>[2x]MSEFNITETYLRFLEEDTEMTMPIAAIEALVTLLRIKTPETAAEMINTIKSSTEELIKSIPNSVSLRAGCDIFMRFVLRNLHLYGDWENCKQHLIENGQLFVSRAKKSRNKIAEIGVDFIADDDIILVHGYSRAVFSLLNHAANKFIRFRCVVTESRPSKQGNQLYTLLEQKGIPVTLIVDSAVGAVIDKVDKVFVGAEGVAESGGIINLVGTYSVGVLAHNARKPFYVVTESHKFVRMFPLSSDDLPMAGPPLDFTRRTDDLEDALRGPTIDYTAQEYITALITDLGVLTPSAVSEELIKMWYD;>[2x]MSSQAFTSVHPNAATSDVNVTIDTFVAKLKRRQVQGSYAIALETLQLLMRFISAARWNHVNDLIEQIRDLGNSLEKAHPTAFSCGNVIRRILAVLRDEVEEDTMSTTVTSTSVAEPLISSMFNLLQKPEQPHQNRKNSSGSSSMKTKTDYRQVAIQGIKDLIDEIKNIDEGIQQIAIDLIHDHEILLTPTPDSKTVLKFLITARERSNRTFTVLVTEGFPNNTKNAHEFAKKLAQHNIETLVVPDSAVFALMSRVGKVIIGTKAVFVNGGTISSNSGVSSVCECAREFRTPVFAVAGLYKLSPLYPFDVEKFVEFGGSQRILPRMDPRKRLDTVNQITDYVPPENIDIYITNVGGFNPSFIYRIAWDNYKQIDVHLDKNKA;>[2x]MSIQAFVFCGKGSNLAPFTQPDFPFQTQNKDSTAATSGDKLNELVNSALDSTVINEFMQHSTRLPKALLPIGNRPMIEYVLDWCDQADFKEISVVAPVDEIELIESGLTSFLSLRKQQFELIYKALSNSNHSHHLQDPKKINFIPSKANSTGESLQKELLPRINGDFVILPCDFVTDIPPQVLVDQFRNRDDNNLAMTIYYKNSLDSSIDKKQQQKQKQQQFFTVYSENEDSERQPILLDVYSQRDVTKTKYLQIRSHLLWNYPNLTVSTKLLNSFIYFCSFELCQLLKLGPQSMSRQASFKDPFTGNQQQQNPPTTDDDEDRNHDDDDDYKPSATSIQPTYFKKKNDLILDPINCNKSLSKVFRDLSRRSWQHSKPREPIGIFILPNETLFIRANNLNAYMDANRFVLKIKSQTMFTKNIQIQSAAIGADAIVDPKCQISAHSNVKMSVLGTQANIGSRCRVAGSLLFPGVHLGDEVILENCIIGPMAKIGSKCKLSNCYIEGHYVVEPKNNFKGETLANVYLDEDEEDELIYDDSVIAGESEIAEETDSDDRSDEDSDDSEYTDEYEYEDDGLFER;>MSESEAKSRSATPPSKAKQATPTTTAAANGEKKLTNKELKELKKQEKAAKRAAMKQANGISIEQQQQQAQMKKEKKQLQREQQQKREQKQKNANKKKQNERNVKKSTLFGHLETTEERRATILALTSAVSSPKTSRITAAGLMVPVVASALSGSNVLTASSLMPVGPNASSTVSASAPASTTTTLPASSAALSAGTSSASTNTPTAIQQEIASSNASDVAKTLASISLEAGEFNVIPGISSVIPTVLEQSFDNSSLISSVKELLLNKDLIHPSILLLTSHLAHYKIVGSIPRCIAMLEVFQIVIKDYQTPKGTTLSRNLTSYLSHQIDLLKKARPLSVTMGNAIRWLKQEISLIDPSTPDKAAKKDLCEKIGQFAKEKIELADQLIIDNASTQIEESTTIVTYGSSKVLTELLLHNAISLKKNIKVIVVDSRPLFEGRKMAETLRNAGVNVMYALITSLDTIFNMDVDYVFLGAHSILSNGFLYSRAGTAMLAMSAKRRNIPVLVCCESLKFSQRVQLDSVTFNELADPNDLVNIDYENPVERRGNKGALLNQFIKERKFEKKKLAMENKPKGNKIGGKKGSEGESKDASNEEDSNSKNILDGWQELPSLNIVNILYDLTPPEYIKKVITEFGALPPSSVPVILREYKGSA[2x];>[2x]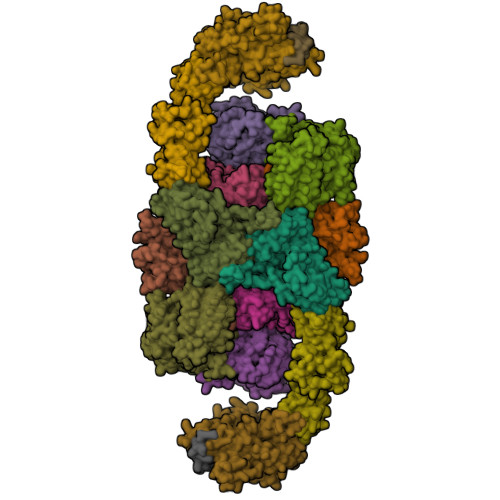MAGKKGQKKSGLGNHGKNSDMDVEDRLQAVVLTDSYETRFMPLTAVKPRCLLPLANVPLIEYTLEFLAKAGVHEVFLICSSHANQINDYIENSKWNLPWSPFKITTIMSPEARCTGDVMRDLDNRGIITGDFILVSGDVLTNIDFSKMLEFHKKMHLQDKDHISTMCLSKASTYPKTRTIEPAAFVLDKSTSRCIYYQDLPLPSSREKTSIQIDPELLDNVDEFVIRNDLIDCRIDICTSHVPLIFQENFDYQSLRTDFVKGVISSDILGKHIYAYLTDEYAVRVESWQTYDTISQDFLGRWCYPLVLDSNIQDDQTYSYESRHIYKEKDVVLAQSCKIGKCTAIGSGTKIGEGTKIENSVIGRNCQIGENIRIKNSFIWDDCIIGNNSIIDHSLIASNATLGSNVRLNDGCIIGFNVKIDDNMDLDRNTKISASPLKNAGSRMYDNESNEQFDQDLDDQTLAVSIVGDKGVGYIYESEVSDDEDSSTEACKEINTLSNQLDELYLSDDSISSATKKTKKRRTMSVNSIYTDREEIDSEFEDEDFEKEGIATVERAMENNHDLDTALLELNTLRMSMNVTYHEVRIATITALLRRVYHFIATQTLGPKDAVVKVFNQWGLLFKRQAFDEEEYIDLMNIIMEKIVEQSFDKPDLILFSALVSLYDNDIIEEDVIYKWWDNVSTDPRYDEVKKLTVKWVEWLQNADEESSSEEE;>MSTSHCRFYENKYPEIDDIVMVNVQQIAEMGAYVKLLEYDNIEGMILLSELSRRRIRSIQKLIRVGKNDVAVVLRVDKEKGYIDLSKRRVSSEDIIKCEEKYQKSKTVHSILRYCAEKFQIPLEELYKTIAWPLSRKFGHAYEAFKLSIIDETVWEGIEPPSKDVLDELKNYISKRLTPQAVKIRADVEVSCFSYEGIDAIKDALKSAEDMSTEQMQVKVKLVAAPLYVLTTQALDKQKGIEQLESAIEKITEVITKYGGVCNITMPPKAVTATEDAELQALLESKELDNRSDSEDDEDESDDE[2x];>[2x]MSDLQDQEPSIIINGNLEPVGEPDIVEETEVVAQETQETQDADKPKKKVAFTGLEEDGETEEEKRKREFEEGGGLPEQPLNPDFSKLNPLSAEIINRQATINIGTIGHVAHGKSTVVRAISGVQTVRFKDELERNITIKLGYANAKIYKCQEPTCPEPDCYRSFKSDKEISPKCQRPGCPGRYKLVRHVSFVDCPGHDILMSTMLSGAAVMDAALLLIAGNESCPQPQTSEHLAAIEIMKLKHVIILQNKVDLMREESALEHQKSILKFIRGTIADGAPIVPISAQLKYNIDAVNEFIVKTIPVPPRDFMISPRLIVIRSFDVNKPGAEIEDLKGGVAGGSILNGVFKLGDEIEIRPGIVTKDDKGKIQCKPIFSNIVSLFAEQNDLKFAVPGGLIGVGTKVDPTLCRADRLVGQVVGAKGHLPNIYTDIEINYFLLRRLLGVKTDGQKQAKVRKLEPNEVLMVNIGSTATGARVVAVKADMARLQLTSPACTEINEKIALSRRIEKHWRLIGWATIKKGTTLEPIA;>MSSDLAAELGFDPALKKKKKTKKVIPDDFDAAVNGKENGSGDDLFAGLKKKKKKSKSVSADAEAEKEPTDDIAEALGELSLKKKKKKTKDSSVDAFEKELAKAGLDNVDAESKEGTPSANSSIQQEVGLPYSELLSRFFNILRTNNPELAGDRSGPKFRIPPPVCLRDGKKTIFSNIQDIAEKLHRSPEHLIQYLFAELGTSGSVDGQKRLVIKGKFQSKQMENVLRRYILEYVTCKTCKSINTELKREQSNRLFFMVCKSCGSTRSVSSIKTGFQATVGKRRRM[2x]> MHHHHHHLPNITILATGGTIAGGGDSATKSNYTVGKVGVENLVNAVPQLKDIANVKGEQVVNIGSQDMNDNVWLTLAKKINTDCDKTDGFVITHGTDTMEETAYFLDLTVKCDKPVVMV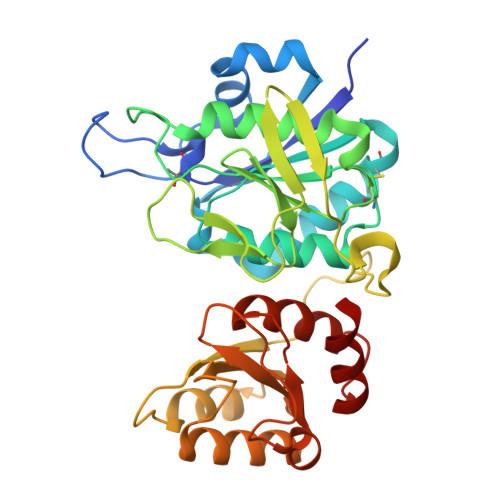GAMRPSTSMSADGPFNLYNAVVTAADKASANRGVLVVMNDTVLDGRDVTMTNTTDVATFKSVNYGPLGYIHNGKIDYQRTPARKHTSDTPFDVSKLNELPKVGIVYNYANASDLPAKALVDAGYDGIVSAGVGNGNLYKSVFDTLATAAKTGTAVVRSSRVPTGATTQDAEVDDAKYGFVASGTLNPQKARVLLQLALTQTKDPQQIQQIFNQY> MEKALKIKQIVVVLIAIAAVAIGYYMFQSITSPAKAVAKQENVVQLASEQPKVEMNKTAPSRFNGKERKVAYLTFDDGPGKYTAELLNTLKQHDAKATFFLIGANVKEFPDLVKRENAEGHYVGMHSMTHNFAKLYKNGEYVNEMKEDQGLIANIIGKSPKLTRPPYGSMPGLNEGLRNKVVEGGFKVWDWTIDSLDWRYNKMPVDAAAAQIAQNVLTNATKPQEVILMHDIHPQSVAAVPAILKGLKEKGYEFEAYHEESHFPVN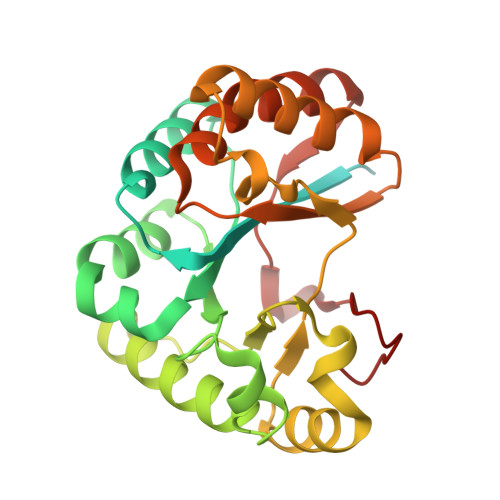FWHDNRM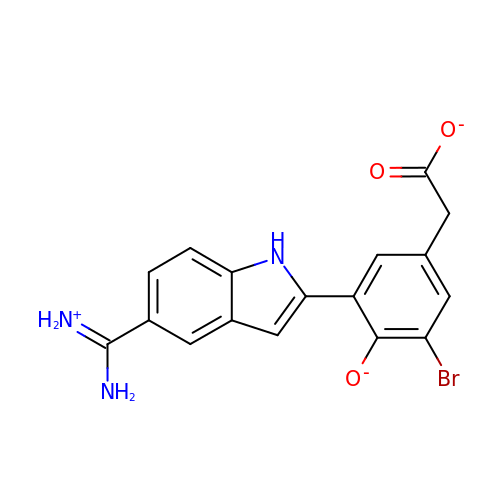(3-{5-[AMINO(IMINIO)METHYL]-1H-INDOL-2-YL}-5-BROMO-4-OXIDOPHENYL)ACETATE | C17 H13 Br N3 O3 | VIZNZQTZRMTYPZ-UHFFFAOYSA-M> MAGQLLFANFNQDNTSLAVGSKSGYKFFSLSSVDKLEQIYECTDTEDVCIVERLFSSSLVAIVSLKAPRKLKVCHFKKGTEICNY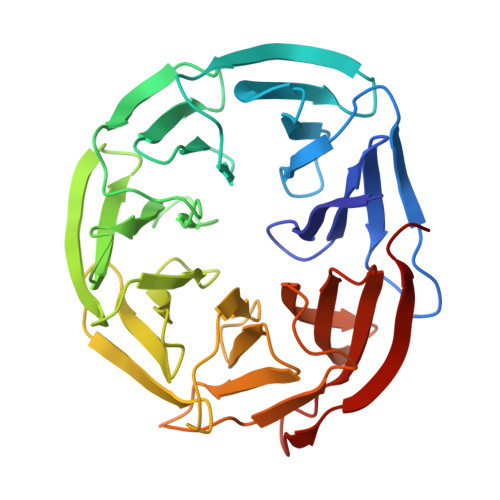SYSNTILAVKLNRQRLIVCLEESLYIHNIRDMKVLHTIRETPPNPAGLCALSINNDNCYLAYPGSATIGEVQVFDTINLRAANMIPAHDSPLAALAFDASGTKLATASEKGTVIRVFSIPEGQKLFEFRRGVKRCVSICSLAFSMDGMFLSASSNTETVHIFKLETVGSGSFNQGRAFATVRLPFCGHKNICSLATIQKIPRLLVGAADGYLYMYNLDPQEGGECALMKQHRLDGSLET> MIFSVDKVRADFPVLSREVNGLPLAYLDSAASAQKPSQVIDAEAEFYRHGYAAVHRGIHTLSAQATEKMENVRKRASLFINARSAEELVFVRGTTEGINLVANSWGNSNVRAGDNIIISQMEHHANIVPWQMLCARVGAELRVIPLNPDGTLQLETLPTLFDEKTRLLAITHVSNVLGTENPLAEMITLAHQHGAKVLVDGAQAVMHHPVDVQALDCDFYVFSGHKLYGPTGI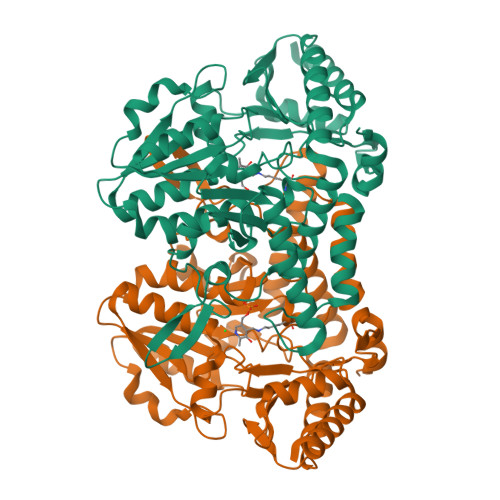GILYVKEALLQEMPPWEGGGSMIATVSLSEGTTWTKAPWRFEAGTPNTGGIIGLGAALEYVSALGLNNIAEYEQNLMHYALSQLESVPDLTLYGPQNRLGVIAFNLGKHHAYDVGSFLDNYGIAVRTGHHCAMPLMAYYNVPAMCRASLAMYNTHEEVDRLVTGLQRIHRLLG Sulfur, essential to many biomolecules such as sulfur-containing amino acids and cofactors including iron-sulfur cluster, is usually mobilized from cysteine by the pyridoxal 5′-phosphate- (PLP-) dependent enzyme of cysteine desulfurase (CDS). We determined the crystal structures of CDS from Thermococcus onnurineus NA1 (ToCDS), which include native internal aldimine (NAT), gem-diamine (GD) with alanine, internal aldimine structure with existing alanine (IAA), and internal aldimine with persulfide-bound Cys356 (PSF) structures. ToCDS belongs to class II CDS based on the primary and tertiary structures and showed the highest similarity with EcSufS. ToCDS is a PLP-dependent enzyme and the crystallographic snapshots of catalytic intermediates of ToCDS showed the conserved dihedral angle rotation of Schiff-base linkage relative to the PLP pyridine ring as shown in EcNifS_CsdB and XometC, which implies the PLP-dependent catalytic mechanism of ToCDS is well conserved.

In crystals II and III, three protomers of GD structure were determined, which showed the clear electron densities of PLP-bound alanine, PLP, and Schiff-base linkage bonds. The persulfide group was removed from substrate cysteine and transferred to Cys356. When we superimposed the ToCDS GD structure into the ToCDS NAT structure, the conformations of the PLP pyridine ring and His114 of both structures were well conserved. However, no tilting of the PLP pyridine ring and His114 was observed in ToCDS. The dihedral angle between the PLP pyridine ring and Schiff-base linkage bond with Lys216 (internal dihedral angle) in the ToCDS GD structure got wider than that in the ToCDS NAT structure by almost 20°. The dihedral angle between the PLP pyridine ring and the Schiff-base linkage with alanine (external dihedral angle) was found to be narrower than the inner dihedral angle. Two amino groups of Lys216 and product alanine had the similar distances of approximate 2.9 Å with the hydroxyl group in an equilateral triangle form. The internal dihedral angle of ToCDS changed from 45° in the NAT structure to 66° in the GD structure on average. In our understanding, the steric hindrance from the incoming substrate amino group of cysteine pushed away the Schiff-base linkage amino group of Lys216 without tilting the PLP pyridine ring due to the tight binding. In the GD structure, the distance between the alanine amino group and the alanine-attached PLP carbon atom decreased as the substrate approached the PLP keeping the same external dihedral angle.

>[2x]MHHHHHHSSENLYFQGHMASMRIPEDVRKDIPLTNEVIYFDNTATSLTPKPVVEAMDEYYLKYRANVHRGVHRLSQMATHKYEESRKIVADFIGAKFEEIVFTKNTSESLNLVALGLGHIFKRGDKIVTTPYEHHSDLLPWQRLATKLGLKLEFIEGDDEGNLDLSDAEKKIKGAKLVAVQHVSNALGVIHEVEELGKIAKDEGAIFVVDAAQSAGHMEVNVKKLHADFLAFSGHKGPMGPTGIGVLYIREEFFDTFEPPLIGGGTIEDVSLDGYKLTEPPERFEAGTPNIGGAIGLAAGIRYIERIGLGRIERQEHKLVKRTTEGLDELEVPWYGPRNLKKHAGVVSFNVPGLHPHDVAAILDDHSIMVRSGHHCALPVMKKLGINGTVRASFHVYNSLEEVETFLGVMEELVKGLKT>MNDVNRIRTDIINVAKTFGAEYSEKVLDEVFQVFGEQFADNSFMIRTSNKQPDKLGCYFRYHEEDESQLGLAWDIARKSGLLSDQGRPVDQLIPEICETFPIMADGVDFDVKHGLAKIWQSIKGVVPVQDAFKLSLPASVTTHSDFLKNHHLDALYAFGIDYHHSSVNLYFDTYHPKHHTSEYYKNLLQDLQFQPPSDELLELLTNNGEIALTFNFASPRIERLCFYLPFLNREAVPQNLLNPLLKKYINEA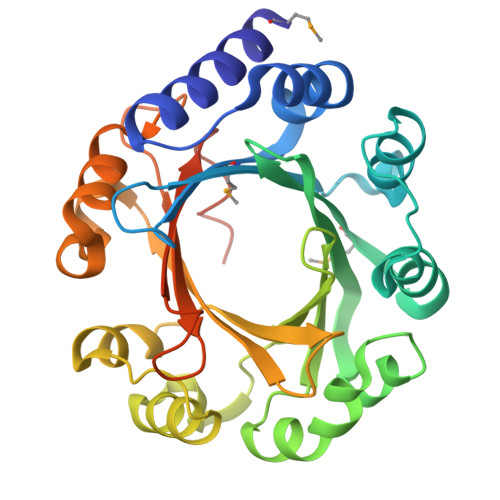PALVDNPGFILGWSFGPQGGKGTYTKVDVDYHGRTVPLFMKVHSQPLPKAADFALAQ[2x]> MAGASVKVAVRVRPFNSREMSRDSKCIIQMSGSTTTIVNPKQPKETPKSFSFDYSYWSHTSPEDINYASQKQVYRDIGEEMLQHAFEGYNVCIFAYGQTGAGKSYTMMGKQEKDQQGIIPQLCEDLFSRINDTTNDNMSYSVEVSYMEIYCERVRDLLNPKNKGNLRVREHPLLGPYVEDLSKLAVTSYNDIQDLMDSGNKPRTVAATNMNETSSRSHAVFNIIFTQKRHDAETNITTEKVSKISLVDLAGSERADSTGAKGTRLKEGANINKSLTTLGKVISALAEMDSGPNKNKKKKKTDFIPYRDSVLTWLLRENLGGNSRTAMVAALSPAD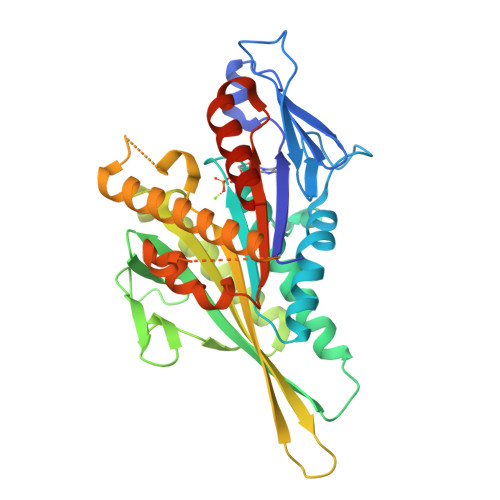INYDETLSTLRYADRAKQIRNTVSVNHHHHH>MTPIETVTAFIAHWNSGDMEAMYDLCAEDVVWHNIPMEPIAGKPAMRAAVEGFMANVSQCDWQVHAIAANGATVLTERTDGFTFTNGRRATIRVMGTFECD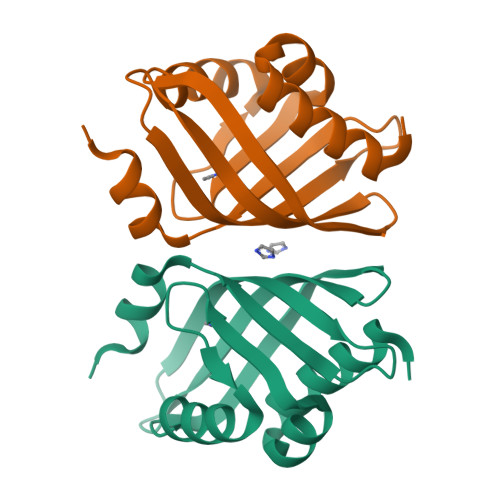AERRIIAWRDYFDMLEFQREFAGA[2x]> GS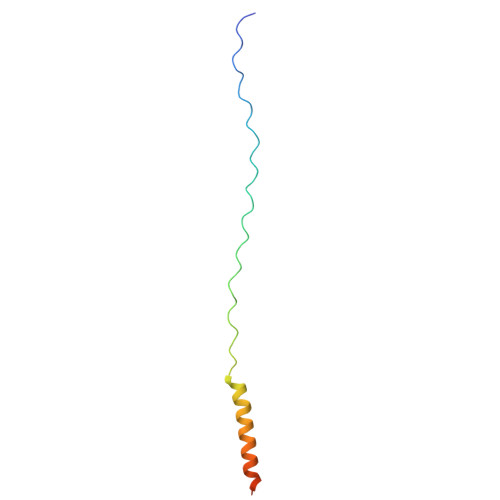GPPGPPGPPGPPGARGQAGVMGFPGPPGPPGPPGRDATDQHIVDVALKMLQEQLAEVAVSAKREALGAV> MQSFSAAAPAASGDFSHITRNTVWGLWNEGNLFSLSVPELAFFLQEHCRVANVDPRAKKSALVRQVEEILSAEQQASATVPQEDNPHAIVVTDYDRAEDALEEADEYGDWGAEPGFEDRRELDFMELSPGRMGERYDPLSPRAFQLLHSETATDVGIASIDPSKLPGQSKVKNALAAIHVAPNDANKMRFRMAFEWCLMNIWNMNMPGELNIGAGKALYYRSVAKQNRNVMPLWTVQKHLYAQHPYAWFAIASESNVAAMESLAAALNMSIQQERTTSYKVTIRRMAEFFDCELNGQLKCTMMNKPWDRFFVSHYIRSKMPDLRYVVRARHPIKKRIADAYLEADILRSTRDSVQSVLSPELGDVVYCCERVVRKWAKKTATGVTLQLVETKRT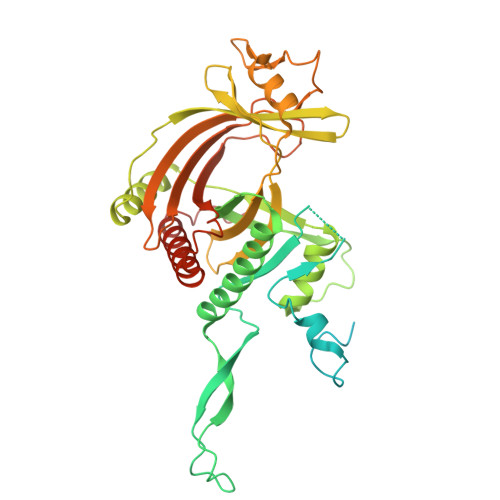PLIITKAGDEGERLEYEWIVPLPQQAERIDIAALTDELWEYGNKLAAALEEGMEELMVHTMTAVSAY>[4x]MAHHHHHHMSQALRIVFAGTPEFAAEHLKALLDTPHRIVAVYTQPDRPAGRGQKLMPSAVKSLALEHGLPVMQPQSLRNAEAQAELAALRADLMVVVAYGLILPQAVLDIPR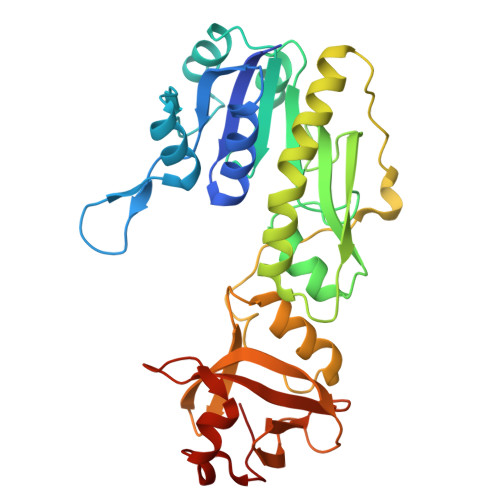LGCINSHASLLPRWRGAAPIQRAVEAGDAESGVTVMQMEAGLDTGPMLLKVSTPISAADTGGSLHDRLAALGPKAVIEAIAGLAAGTLHGEIQDDALATYAHKLNKDEARLDWSRPAVELERQVRAFTPWPVCHTSLADAPLKVLGASLGQGSGAPGTILEASRDGLLVACGEGALRLTRLQLPGGKPLAFADLYNSRREQFAAGQVLGQ>[12x]MEDTMTMPSHAQLKAYFEEARDANEEYRKEAFIDRDYFDGHQWTEEELQKLEARKQPATYFNEVKLSIRGLVGVFEQGDSDPRAWPRNPQDEDSADIATKALRYVKDYSEWSDERSRAALNYFVEGTCAAIVGVDENGRPEIEPIRFEEFFHDPRSRELDFSDARFKGVAKWRFADEVGMEYGIKGEIDGALDGDSEGLSIGGDTFGDRPDGKISSWIDSKLRRVFVVEMYVRWNGVWIRALFWGRGILEMSVSAYLDRNGKPTCPIEARSCYIDRENRR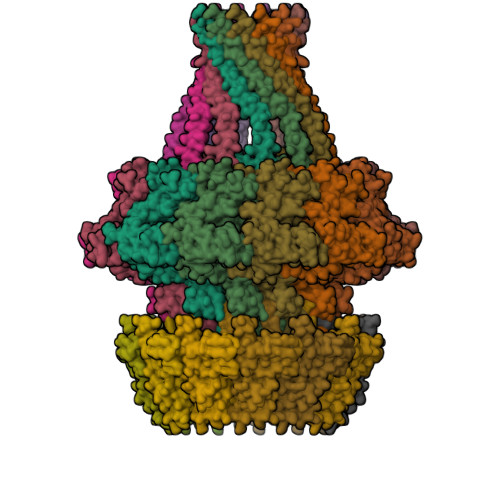YGEVRDLRSPQDAINKRESKLLHMLNNRQAIATNPEYAYNSDAEMVRKEMSKPDGIIPPGWQPASMTDLANGQFALLSSAREFIQRIGQNPSVLAAQSASASGRAQLARQQAGMVDSAMALNGLRRFELAVYRQAWLRCRQFWKAPDYIRVTDDEGAPQFVGINQPIKGPPQPVLNEMGQVVIAEPILGYENALAELDVDINIDAVPDTANLAQEQFLQLTELARLYGPQEVPFDDLLELSSMPEKTKLIAKRRERSEQMAQVQAQQGQMQEQIAMQGAMAEIENTQADTAYLAARAQNEMLKPQIEAFKAGFGAA;>MITCRDIITLGLQQARVVPLGREPKAKEADAGLTVLQSIYDSMFADGPLGPFTEVYATSAYTAQENERIVTNGAAITIPQTITEGNETRKPYDLTAIIVINGAAQENHVFSLGRWQTAHDLTLNSEAPLAERDKAGLAALFAMEFAEMFGAELPPRTTARGFRFKGAISQKLATKRDDPVYY[12x]>RSPRLVGADMPCSGRVEVKHADTWRSVCDSDFSLHAANVLCRELNCGDAISLSVGDHFGKGNGLTWAEKFQCEGSETHLALCPIVQHPEDTCIHSREVGVVCST[2x]

Infection by its etiological agent, PRRS virus (PRRSV), shows a highly restricted tropism of host cells and has been demonstrated to be mediated by an essential scavenger receptor (SR) CD163. CD163 fifth SR cysteine-rich domain (SRCR5) is further proven to play a crucial role during viral infection. In the current study, we prepared recombinant monkey CD163 (moCD163) SRCR5 and human CD163-like homolog (hCD163L1) SRCR8, and determined their crystal structures. After comparison with the previously reported crystal structure of porcine CD163 (pCD163) SRCR5, these structures showed almost identical structural folds but significantly different surface electrostatic potentials.

Additionally, a significantly reduced permissiveness to PRRSV-2, particularly HP-PRRSV, was shown in the PAMs with pCD163 SRCR5 substitution by homologous hCD163L1 SRCR8. MoCD163 SRCR5 was comprised of two antiparallel β-sheets (β1-4, β7 and β5-6) and three helices (a single α-helix α2 and two 310-helices α1, α3), whereas hCD163L1 SRCR8 contained two antiparallel β-sheets (β1-4, β7 and β5-6) and two helices (a single α-helix α1 and a 310-helix α2). A close comparison of moCD163 SRCR5 or hCD163L1 SRCR8 with pCD163 SRCR5 revealed that they shared almost identical structural folds (RMSD = 0.355 Å for 79 matching Cα atoms between moCD163 SRCR5 and pCD163 SRCR5, RMSD = 0.249 Å for 95 matching Cα atoms between hCD163L1 SRCR8 and pCD163 SRCR5). In addition to minor differences in the long loop region, hCD163L1 SRCR8 contained a shorter β4 (Ile842-Ser845) than that of pCD163 SRCR5 (Thr522-Leu527). In contrast, hCD163L1 SRCR8 showed a significantly different surface electrostatic potential from the other two proteins. There were more positively and negatively charged regions in hCD163L1 SRCR8 due to different amino acid contents. Especially, certain regions with the opposed charge were clearly observed, where the acidic residues were replaced by the basic ones. Based on the comparison, we hypothesize that the difference in the surface electrostatic potentials between hCD163L1 SRCR8 and pCD163 SRCR5 may result in reduced cell permissiveness to PRRSV-2 infection, rather than their structural folds. Furthermore, this comparison suggested that the surface electrostatic potential might lead to different cell susceptibility to PRRSV infection between pCD163 and hCD163L1, where pCD163 SRCR5 substitution by homologous hCD163L1 SRCR8 showed a significantly reduced permissiveness to PRRSV-2.> MIKVTIFLLLSIFSFNLYGLELNEKVSIKYGAEQGVGSADSNTKLCSDILKYLYMDEYLSEGDKATFEKKCHNVIGNIRNTFSNKNTIKEGNEFLMSILHMKSLYGNNNNNNAGSESDVTLKSLYLSLKGSQNTEGESEVPSDDEINKTIMNFVKFNKYLLDNSNDIKKVHDFLVLTSQSNENLLPNKEKLFEQIVDQIKYFDEYFFASGGKIKVKKGYLKYNFLDIYKQPVCSAYLHLCSRYYESVSIYIRLKKVFNGIPAFLDKNCRKVKGEEFKKLMDMELKHNHIVERFDKYIISDDLYYVNMKVFDLKNVDKIQVSKIDDINNLNIYEHKETMHLSAKNLSRYIDIKKELNDEKAYKQLMSAIRKYVTTLTKADSDITYFVKQLDDEEIERFLIDLNFFLYNGFLRITEDKHLINADDVSPSYINLYRSNNIVALYILKTQYEENKLSEYRAHKFYRRKRVSNITNDMIKKDFTQTNALTNLPNLDNKKTTEYYLKEYENFVENFQPDLHDIMKLQLFFTMAFKDCNVNQNFTETSKKLWFDLLYAYDKFGWFYIHPNEVINSINKTDFVRHVLVSRNFLLKNNDQLTFLETQVAKIVEIINLSLEVDKSPDSLDFSIPMNFFNHKNGYHVMNDDKLKLLTSYEYIDSIANNYFFLSEYKNDVFRTGNNFKLYFNLPNIYSLAYQLFNELAININVITNVPLKKYLKYNASYAYFTLMNMIGKNHDIYSKGSRFVYASYILGLVFFIESHIDIARLKPKDFFFMKQSLPIIDHVYHKDLKTLKKNCTLLTDFMKINKNSQNYSLTHTEEMIKILGLLTVTLWAKEGKKSVYYDDDVSLYRKLMVSCVFNGGETIQEKLANNIEKSCDISQYGIKSKNLKDMIDINLSIHKWNPAEIEKLAYSFVLSCKMQKLMYKPMNVEKLPLEDYYKLSLAPDMVKTYHCYKLGKQAAELLESIILKKKFVRFRVTDAIDVYDFFYIKKVLSSRIKKEYNEFLQDKRAFEKKELETILNNSPFSEEQTMKLINSYECHWFTSYENFRILWMHASSNLGTGTYLKNFFSELWQNIRFLFKSKLKIRDMEYFSGDISQMNLLDYYSPMVHSESHCQEKMQVLFITLR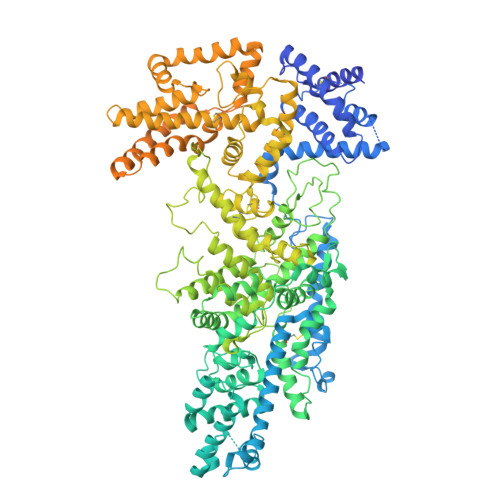DSKEENRSEIAQKVKSAYYQCKLDYYKNHHSDFIHRIHPNDFLNNKVYVLKQPYYLMSNVPLNNPKKVSRLFVTEGTLEYLLLDKINIPECFGPCTKLHFNKVVIKESKQRIYDMTINNALVPEIQPYNRRKYMTIYINEAYIKNIVSDALTSEEIKRHDIQKGNIKICMGKSTYLTEPILTEEHFNLTHKPVYDFSSVKHNLKVFHMKNEHLVSEDPNDDCFINYPLATINLDISDPYKEISEDLIKNLYILKSS>MDLATLLGLIGGFAFVIMAMVLGGSIGMFVDVTSILIVVGGSIFVVLMKFTMGQFFGATKIAGKAFMFKADEPEDLIAKIVEMADAARKGGFLALEEMEINNTFMQKGIDLLVDGHDADVVRAALKKDIALTDERHTQGTGVFRAFGDVAPAMGMIGTLVGLVAMLSNMDDPKAIGPAMAVALLTTLYGAILSNMVFFPIADKLSLRRDQETLNRRLIMDGVLAIQDGQNPRVIDSYLKNYLNEGKRALEIDE[5x];>MDDEDNKCDCPPPGLPLWMGTFADLMSLLMCFFVLLLSFSEMDVLKFKQIAGSMKFAFGVQNQLEVKDIPKGTSIIAQEFRPGRPEPTPIDVIMQQTMDITQQTLEFHEGESERAGGTKRDEGKLTGGQSPETSTQNNESAEADMQQQQSKEMSQEMETLMESIKKALEREIEQGAIEVENLGQQIVIRMREKGAFPEGSAFLQPKFRPLVRQIAELVKDVPGIVRVSGHTDNRPLDSELYRSNWDLSSQRAVSVAQEMEKVRGFSHQRLRVRGMADTEPLLPNDSDENRALNRRVEISIMQGEPLYSEEVPVIQ[2x]

Vibrio spp. are highly motile bacteria responsible for various human diseases, the polar flagella of which are exclusively driven by sodium-dependent stator units (PomAB). The flagellar stator unit uses the transmembrane ion motive force (IMF) to generate mechanical torque to rotate the flagellum, which is employed by many bacteria to direct their locomotion in liquid environment or on viscous surfaces to a favorable niche. PomAB assembles the characteristic bell shape of the stator unit family, with conserved 5:2 subunit stoichiometry and overall architecture. Five PomA molecules arrange pseudo-symmetrically around two PomB, with each PomA subunit comprising four transmembrane helices (TM1-TM4) folded into two radial layers.

The high-resolution PomAB structure was determined in a detergent micelle environment, raising the possibility that detergent molecules could have an impact on the conformation of PomAB, particularly the membrane-facing helices, including the disordered TM1 from two PomA subunits. To clarify this and to better mimic the native environment of the stator unit, we reconstituted VaPomAB into membrane scaffold protein 1D1 (MSP1D1) nanodiscs, as well as full length, non-cleaved VaPomAB into saposin nanodiscs, with E. coli polar lipids, and determined the map resolution, at 3.9 Å and 6.3 Å, respectively. In both cases, we were able to trace all the secondary structure elements of the PomAB complex, except the two PomA TM1 helices. Comparison of the PomAB LMNG structure to the MSP1D1 lipid-reconstituted structure did not reveal major conformational differences (root-mean-square deviation of 0.642 Å, 1,312 Cα atoms aligned) that could arise from detergent artifacts. This indicates that the flexibility of those two TM1 helices in the inactive stator unit is probably intrinsic, which might be functionally important during stator unit activation.> QIASDVEAPPPAPAKVEKHSKKMEEGITVNKFKPKTPYVGRCLLNTKITGDDAPGETWHMVFSHEGEIPYREGQSVGVIPDGEDKNGKPHKLRLYSIASSALGDFGDAKSVSLCVKRLIYTNDAGETIKGVCSNFLCDLKPGAEVKLTGPV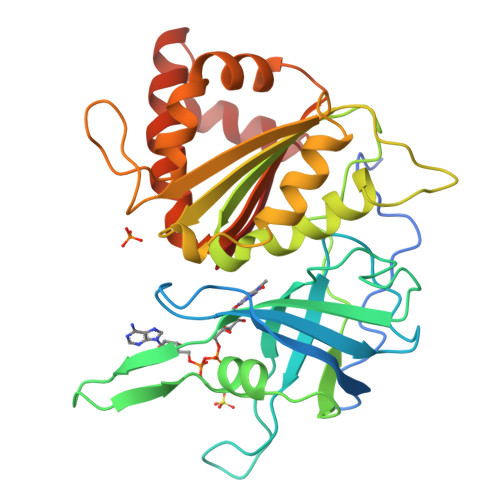GKEMLMPKDPNATIIMLGTGTGIAPFRSFLWKMFFEKHDDYKFNGLAWLFLGVPTSSSLLYKEEFEKMKEKAPDNFRLDFAVSREQTNEKGEKMYIQTRMAQYAVELWEMLKKDNTYVYMCGLKGMEKGIDDIMVSLAAAEGIDWIEYKRQLKKAEQWNVEVY>[2x]MGERPPPKRLTREAMRNYLKERGDQTVLILHAKVAQK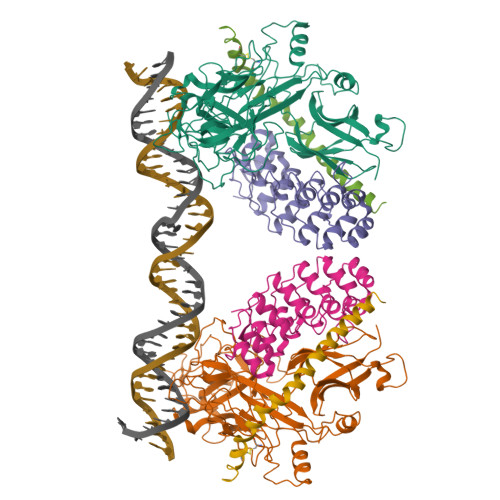SYGNEKRFFCPPPCVYLMGSGWKKKKEQMERDGCSEQESQPCAFIGIGNSDQEMQQLNLEGKNYCTAKTLYISDSDKRKHFMLSVKMFYGNSDDIGVFLSKRIKVISKPSKKKQSLKNADLCIASGTKVALFNRLRSQTVSTRYLHVEGGNFHASSQQWGAFFIHLLDDDESEGEEFTVRDGYIHYGQTVKLVCSVTGMALPRLIIRKVDKQTALLDADDPVSQLHKCAFYLKDTERMYLCLSQERIIQFQATPCPKEPNKEMINDGASWTIISTDKAEYTFYEGMGPVLAPVTPVPVVESLQLNGGGDVAMLELTGQNFTPNLRVWFGDVEAETMYRCGESMLCVVPDISAFREGWRWVRQPVQVPVTLVRNDGIIYSTSLTFTYTPEPHHHHHH;>[2x]GMDVNVRGPDGFTPLMIASCSGGGLETGNSEEEEDAPAVISDFIYQGASLHNQTDRTGETALHLAARYSRSDAAKRLLEASADANIQDNMGRTPLHAAVSADAQGVFQILIRNRATDLDARMHDGTTPLILAARLAVEGMLEDLINSHADVNAVDDLGKSALHWAAAVNNVDAAVVLLKNGANKDMQNNREETPLFLAAREGSYETAKVLLDHFANRDITDHMDRLPRDIAQERMHHDIVRLLDEYNLVRSPQLHG;>GLPRHSAVMERLRRRIELCRRHHSTCEARYEAVSPERLELERQHTFALHQRCIQAKAKRAGKH[2x]>MGHHHHHHMQVADKHELGQLQYSLDYDFQSGQLLVGILQAMGLAALDLGGSSDPYVRVYLLPDKRRRYETKVHRQTLNPHFGETFAFKVPYVELGGRVLVMAVYDFDRFGRNDAIGEVRVPMSSVDLGRPVQAWRELQAAP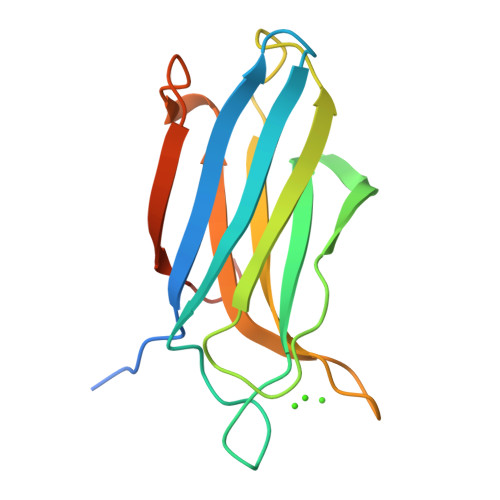REEQEKLGD[2x]> GLEFNSFQHQLRIQDQEFQEGFDGGWCLSVHQP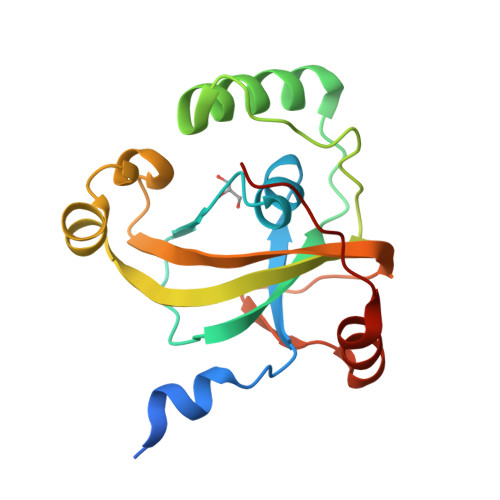WASLLVRGIKRVEGRSWYTPHRGRLWIAATAKKPSPQEVSELQATYRLLRGKDVEFPNDYPSGCLLGCVDLIDCLSQKQFKEQFPDISQESDSPFVFICKNPQEMVVKFPIKGNPKIWKLDSKIHQGAKKGLMKQNKAV> MHHHHHHSSGRENLYFQGVRIITNYGDLKFELFCSQCPKACKNFLALSASGYYKNTIFHKNIKGFIIQGGDPTGTGKGGESIYGRYFDDEIYPELKYDRRGILSMASKGASKKPNTNGSQFFITYSSLPQLNGEYVIFGKLI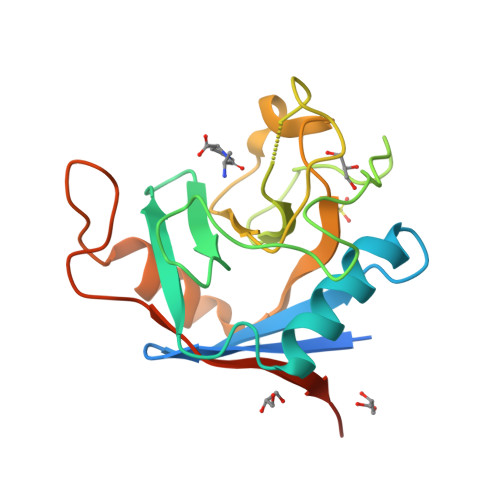DGFETLNTLENCPSDKSHKPIDEIIIKDIVIHSNPIADQEILD>MGSDKIHHHHHHMKPLRKIRLGIVGCGIAARELHLPALKNLSHLFEITAVTSRTRSHAEEFAKMVGNPAVFDSYEELLESGLVDAVDLTLPVELNLPFIEKALRKGVHVICEKPISTDVETGKKVVELSEKSEKTVYIAENFRHVPAFWKAKELVESGAIGDPVFMNWQIWVGMDENNKYVHTDWRKKPKHVGGFLSDGGVHHAAA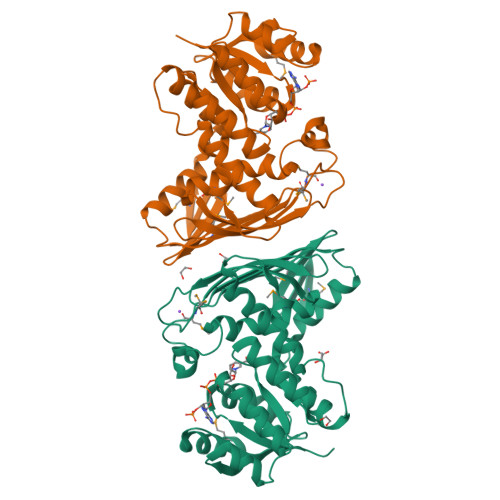MRLILGEIEWISAVAKDLSPLLGGMDFLSSIFEFENGTVGNYTISYSLKGNERFEITGTKGKISISWDKIVLNEEEMKVPQENSYQKEFEDFYQVVAEGKPNDLGSPVQALKDLAFIEACVRSAGNKVFVSSLL[2x]> MEKETGPEVDDSKVTYDTIQSKVLKAVIDQAFPRVKEYSLNGHTLPGQVQQFNQVFINNHRITPEVTYKKINETTAEYLMKLRDDAHLINAEMTVRLQVVDNQLHFDVTKIVNHNQVTPGQKIDDESKLLSSISFLGNALVSVSSDQTGAKFDGATMSNNTHVSGDDHIDVTNPMKDLAKGYMYGFVSTDKLAAGVWSNSQNSYGGGSNDWTRLTAYKETVGNANYVGIHSSEWQWEKAYKGIVFPEYTKELPSAKVVITEDANADKNVDWQDGAIAYRSIMNNPQGWEKVKDITAYRIAMNFGSQAQNPFLMTLDGIKKINLHTDGLGQGVLLKGYGSEGHDSGHLNYADIGKRIGGVEDFKTLIEKAKKYGAHLGIHVNASETYPESKYFNEKILRKNPDGSYSYGWNWLDQGINIDAAYDLAHGRLARWEDLKKKLGDGLDFIYVDVWGNGQSGDNGAWATHVLAKEINKQGWRFAIQWGHGGEYDSTFHHWAADLTYGGYTNKGINSAITRFIRNHQKDAWVGDYRSYGGAANYPLLGGYSMKDFEGWQGRSDYNGYVTNLFAHDVMTKYFQHFTVSKWENGTPVTMTDNGSTYKWTPEMRVELVDADNNKVVVTRKSNDVNSPQYRERTVTLNGRVIQDGSAYLTPWNWDANGK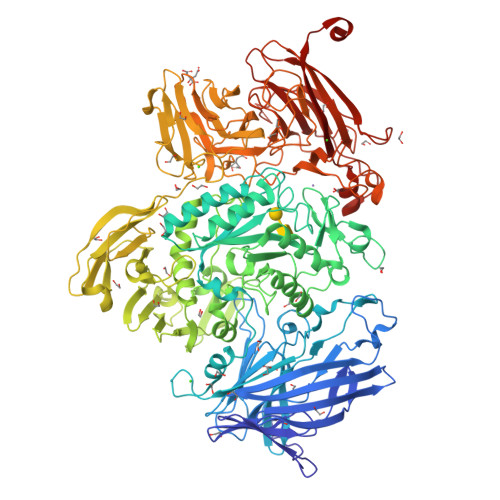KLSTDKEKMYYFNTQAGATTWTLPSDWAKSKVYLYKLTDQGKTEEQELTVKDGKITLDLLANQPYVLYRSKQTNPEMSWSEGMHIYDQGFNSGTLKHWTISGDASKAEIVKSQGANDMLRIQGNKEKVSLTQKLTGLKPNTKYAVYVGVDNRSNAKASITVNTGEKEVTTYTNKSLALNYVKAYAHNTRRNNATVDDTSYFQNMYAFFTTGADVSNVTLTLSREAGDEATYFDEIRTFENNSSMYGDKHDTGKGTFKQDFENVAQGIFPFVVGGVEGVEDNRTHLSEKHDPYTQRGWNGKKVDDVIEGNWSLKTNGLVSRRNLVYQTIPQNFRFEAGKTYRVTFEYEAGSDNTYAFVVGKGEFQSGRRGTQASNLEMHELPNTWTDSKKAKKATFLVTGAETGDTWVGIYSTGNASNTRGDSGGNANFRGYNDFMMDNLQIEEITLTGKMLTHHHHHH> MHLNPAEKEKLQIFLASELLLRRKARGLKLNYPEAVAIITSFIMEGARDGKTVAMLMEEGKHVLTRDDVMEGVPEMIDDIQAEATFPDGTKLVTVHNPIS;> MSNNNYIVPGEYRVAEGEIEINAGREKTTIRVSNTGDRPIQVGSHIHFVEVNKELLFDRAEGIGR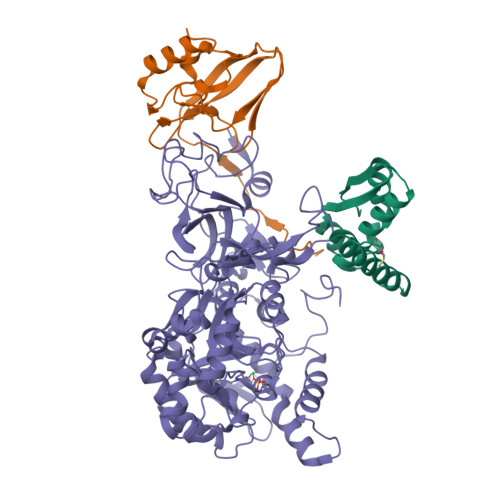RLNIPSGTAARFEPGEEMEVELTELGGNREVFGISDLTNGSVDNKELILQRAKELGYKGVE;> MKINRQQYAESYGPTVGDEVRLADTDLWIEVEKDYTTYGDEVNFGGGKVLREGMGENGTYTRTENVLDLLLTNALILDYTGIYKADIGVKDGYIVGIGKGGNPDIMDGVTPNMIVGTATEVIAAEGKIVTAGGIDTHVHFINPDQVDVALANGITTLFGGGTGPAEGSKATTVTPGPWNIEKMLKSTEGLPINVGILGKGHGSSIAPIMEQIDAGAAGLKIHEDWGATPASIDRSLTVADEADVQVAIHSDTLNEAGFLEDTLRAINGRVIHSFHVEGAGGGHAPDIMAMAGHPNVLPSSTNPTRPFTVNTIDEHLDMLMVCHHLKNNIPEDVAFADSRIRPETIAAEDILHDLGIISMMSTDALAMGRAGEMVLRTWQTADKMKKQRGPLAEEKNGSDNFRLKRYVSKYTINPAIAQGIAHEVGSIEEGKFADLVLWEPKFFGVKADRVIKGGIIAYAQIGDPSASIPTPQPVMGRRMYGTVGDLIHDTNITFMSKSSIQQGVPAKLGLKRRIGTVKNCRNIGKKDMKWNDVTTDIDINPETYEVKVDGEVLTCEPVKELPMAQRYFLF N-(propan-2-yl)pyridin-3-amine | C8 H12 N2 | 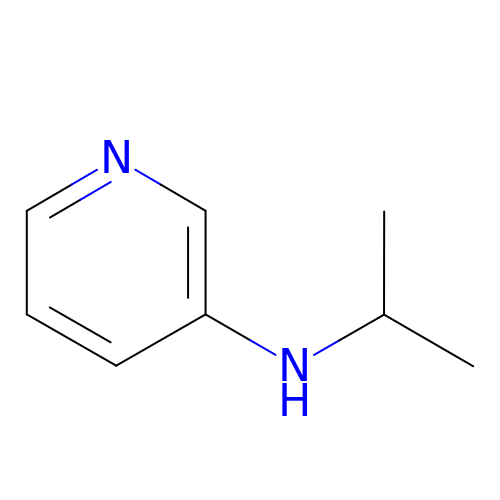KJSHRGNATIWUSZ-UHFFFAOYSA-N>MGLISEEDKRIIKEEFFSKMVNPVKLIVFIGKEHCQYCDQLKQLVQELSELTDKLSYEIVDFDTPEGKELAEKYRIDRAPATTITQDGKDFGVRYFGIPAGHEFAAFLEDIVDVSKGDTDLMQDSKEEVSKIDKDVRILIFVTPTCPY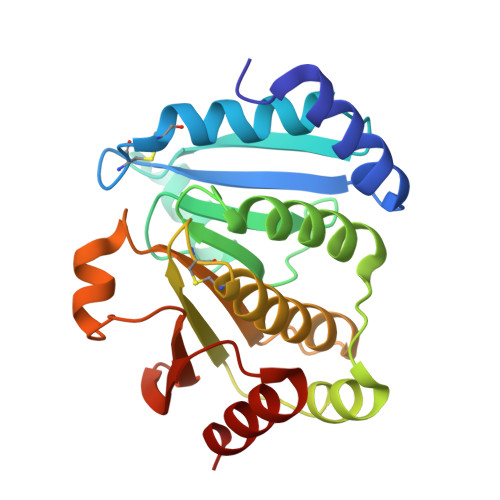CPLAVRMAHKFAIENTKAGKGKILGDMVEAIEYPEWADQYNVMAVPKIVIQVNGEDKVQFEGAYPEKMFLEKLLSALS[8x]>[2x]SMTDQAFVTLTTNDAYAKGALVLGSSLKQHRTTRRLVVLATPQVSDSMRKVLETVFDEVIMVDVLDSGDSAHLTLMKRPELGVTLTKLHCWSLTQYSKCVFMDADTLVLANIDDLFDREELSAAPDPGWPDCFNSGVFVYQP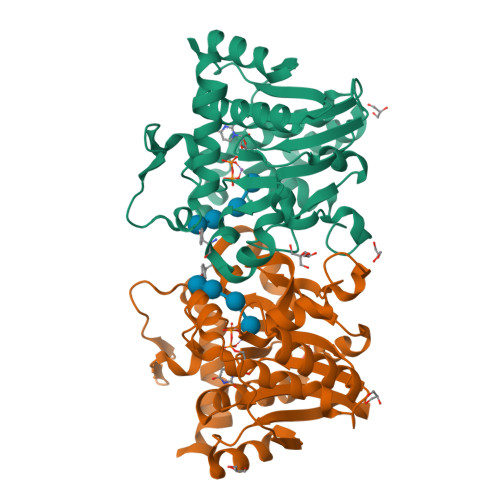SVETYNQLLHLASEQGSFDGGDQGILNTFFSSWATTDIRKHLPFIYNLSSISIYSYLPAFKVFGASAKVVHFLGRVKPWNYTYDPKTKSVKSEAHDPNMTHPEFLILWWNIFTTNVLPLLQ> SEFVPPPECPVFEPSWEEFTDPLSFIGRIRPLAEKTGICKIRPPKDWQPPFACEVKSFRFTPRVQRLNELEAMTRVRLDFLDQLAKFWELQGSTLKIPVVERKILDLYALSKIVASKGGFEMVTKEKKWSKVGSRLGYLPGKGTGSLLKSHYERILYPYELFQSGVSLMGVQM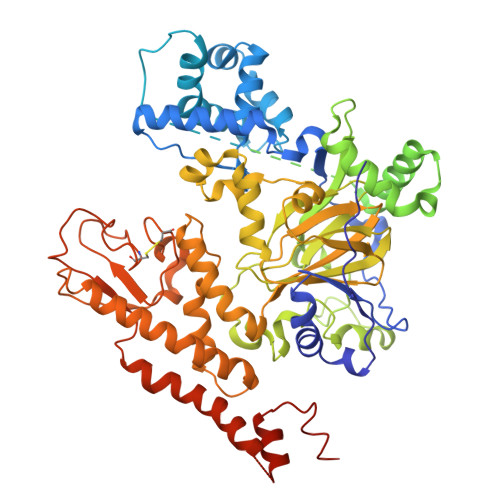PNLDLKEKVEPEVLSTDTQTSPEPGTRMNILPKRTRRVKTQSESGDVSRNTELKKLQIFGAGPKVVGLAMGTKDKEDEVTRRRKVTNRSDAFNMQMRQRKGTLSVNFVDLYVCMFCGRGNNEDKLLLCDGCDDSYHTFCLIPPLPDVPKGDWRCPKCVAEECSKPREAFGFEQAVREYTLQSFGEMADNFKSDYFNMPVHMVPTELVEKEFWRLVSSIEEDVIVEYGADISSKDFGSGFPVKDGRRKILPEEEEYALSGWNLNNMPVLEQSVLAHINVDISGMKVPWLYVGMCFSSFCWHIEDHWSYSINYLHWGEPKTWYGVPSHAAEQLEEVMRELAPELFESQPDLLHQLVTIMNPNVLMEHGVPVYRTNQCAGEFVVTFPRAYHSGFNQGYNFAEAVNFCTADWLPIGRQCVNHYRRLRRHCVFSHEELIFKMAADPECLDVGLAAMVCKELTLMTEEETRLRESVVQMGVLMSEEEVFELVPDDERQCSACRTTCFLSALTCSCNPERLVCLYHPTDLCPCPMQKKCLRYRYPLEDLPSLLYGVKVRAQSYDTWVSRVTEALSANFNHKKDLIELRVMLEDAEDRKYPENDLFRKLRDAVKEAETCASVGNS>[2x]MNSVGFYGKLAGRGDFVSRGLPNTFVEPWDAWLAS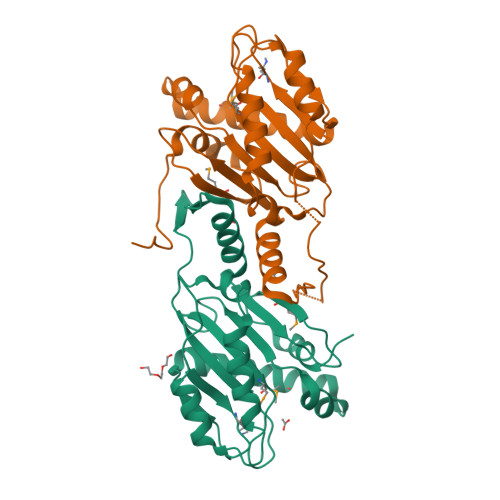GMRASQDELGAAWLDAYLTSPLWRFAIAPGLLGGEAVTGVVMPSIDRVGRYFPLTVACLLPANADLGGLVGGDDGWFEQVESLLLSTLEPEAEVEAFEQAVAQLPAPPCGPRIEQSLISGNLLRSEAVTPAQRLAALAQHACDGASHWWGRGSARISAGLMRYQGLPPAPAFGRFLTGEGEVIPLFPGIPG> APDQDEIQRLPGLAKQPSFRQYSGYLKGSGSKHLHYWFVESQKDPENSPVVLWLNGGPGCSSLDGLLTEHGPFLVQPDGVTLEYNPYSWNLIANVLYLESPAGVGFSYSDDKFYATNDTEVAQSNFEALQDFFRLFPEYKNNKLFLTGESYAGIYIPTLAVLVMQDPSMNLQGLAVGNGLSSYEQNDNSLVYFAYYHGLLGNRLWSSLQTHCCSQNKCNFYDNKDLECVTNLQEVARIVGNSGLNIYNLYAPCAGGVPSHFRYEKDTVVVQDLGNIFTRLPLKRMWHQALLRSGDKVRMDPPCTNTTAASTYLNNPYVRKAL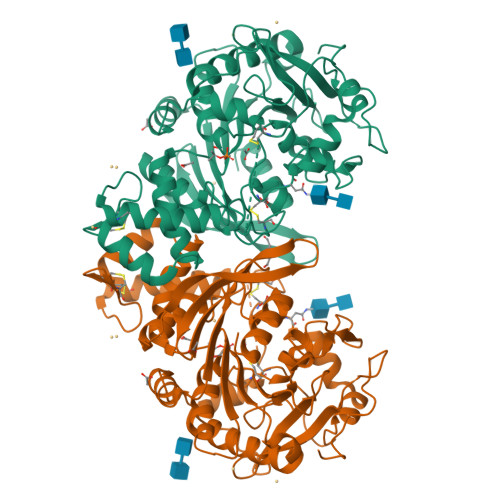NIPEQLPQWDMCNFLVNLQYRRLYRSMNSQYLKLLSSQKYQILLYNGDVDMACNFMGDEWFVDSLNQKMEVQRRPWLVKYGDSGEQIAGFVKEFSHIAFLTIKGAGHMVPTDKPLAAFTMFSRFLNKQPYHHHHHH> MNITKPFPLPTGYFDIPLGL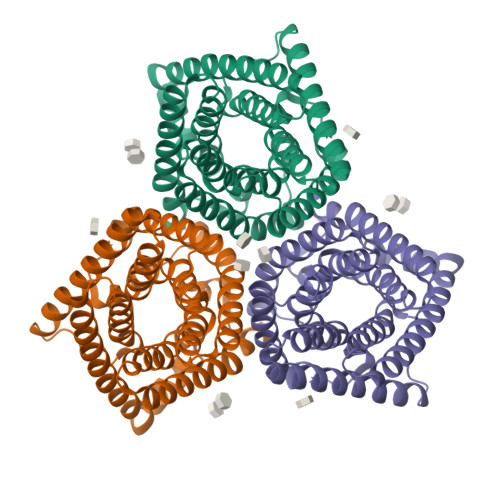AALSLAWFHLENLFPAARMVSDVLGIVASAVWILFILMYAYKLRYYFEEVRAEYHSPVRFSFIALIPITTMLVGDILYRWNPLIAEVLIWIGTIGQLLFSTLRVSELWQGGVFEQKSTHPSFYLPAVAANFTSASSLALLGYHDLGYLFFGAGMIAWIIFEPVLLQHLRISSLEPQFRATMGIVLAPAFVCVSAYLSINHGEVDTLAKILWGYGFLQLFFLLRLFPWIVEKGLNIGLWAFSGGLASMANSATAFYHGNVLQGVSIFAFVFSNVMIGLLVLMTIYKLTKGQFFLK>[2x]MLSFLRSTGRPERRRASLPALLLFTAALVASGLTAAPAAQAADNPYQRGPDPTNASIEAATGPFAVGTQPIVGASGFGGGQIYYPTDTSQTYGAVVIVPGFISVWAQLAWLGPRLASQGFVVIGIETSTITDLPDPRGDQALA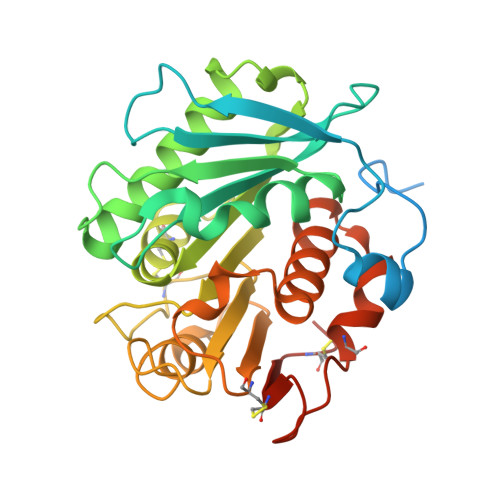ALDWATTRSPVRSRIDRTRLAAAGWSMGGGGLRRAACQRPSLKAIVGMAPWNTEKNWSCVTVPTLFFGGSSDAVASPNDHAKPFYNSITRAEKDYIELCNADHFFPTSANTTMAKYFISWLKRWVDNDTRYTQFLCPGPSTGLFAPVCASMNTCPFLEHHHHHH>GSHMAEVRGVQRVLFG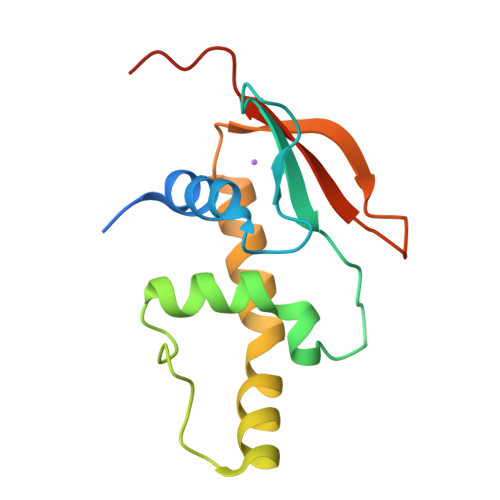DWLLGEVSSGQYEGLQWLNEARTVFRVPWKHFGRRDLDEEDAQIFKAWAVARGRWPPSGVNLPPPEAEAAERRERRGWKTNFRCALHSTGRFILRQDNSGDPVDPHKVYELSRELGSTVGP[3x]> MASRGLDLWLDEHVWKRKQEIGVKGENLLLPDLWLDFLQLSPIFQRKLAAVIACVRRLRTQATVYPEEDMCMAWARFCDPSDIKVVILGQDPYHGGQANGLAFSVAYGFPVPPSLRNIYAELHRSLPEFSPPDHGCLDAWASQGVLLLNTILTVQKGKPGSHADIGWAWFTDHVISLLSERLKACVFMLWGAKAGDKASLINS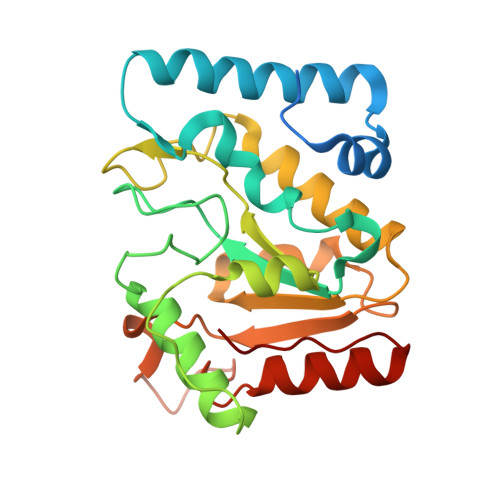KKHLVLTSQHPSPLAQNSTRKSAQQKFLGNNHFVLANNFLREKGLGEIDWRL(4R)-4-hydroxypentanoic acid | C5 H10 O3 | 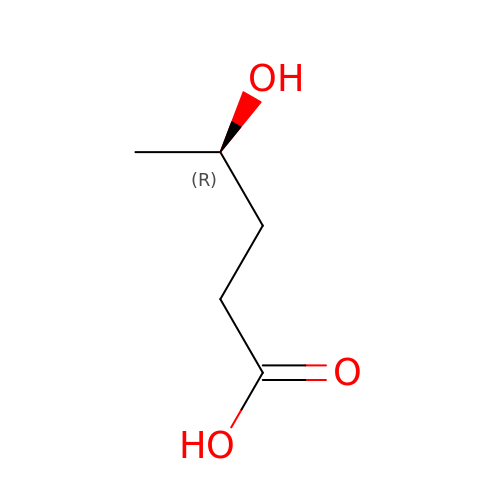FMHKPLXYWVCLME-SCSAIBSYSA-N methyl (2S)-4-hydroxy-3-(4-hydroxyphenyl)-2-[(4-hydroxyphenyl)methyl]-5-oxo-2,5-dihydrofuran-2-carboxylate 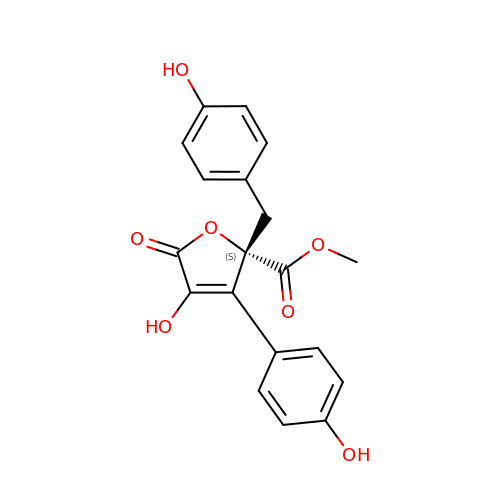| C19 H16 O7 | AEKPZNDJHWFONI-IBGZPJMESA-N6-(cyclohexylamino)pyridine-3-carboxamide 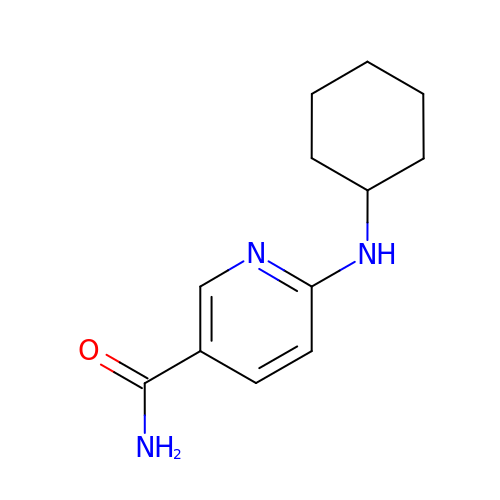| C12 H17 N3 O | DGZXVZSOZVPFDW-UHFFFAOYSA-N> GGSKMEYEWKPDEQGLQQILQLLKESQSPDTTIQRTVQQKLEQLNQYPDFNNYLIFVLTKLKSEDEPTRSLSGLILKNNVKAHFQNFPNGVTDFIKSECLNNIGDSSPLIRATVGILITTIASKGELQNWPDLLPKLCSLLDSEDYNTCEGAFGALQKICEDSAEILDSDVLDRPLNIMIPKFLQFFKHSSPKIRSHAVACVNQFIISRTQALMLHIDSFIENLFALAGDEEPEVRKNVCRALVMLLEVRMDRLLPHMHNIVEYMLQRTQDQDENVALEACEFWLTLAEQPICKDVLVRHLPKLIPVLVNGMKYSDIDIILLKGDVEEDETIPDSEQDIRPRFHRSRTVAQQHDEDGIEEEDDDDDEIDDDDTISDWNLRKCSAAALDVLANVYRDELLPHILPLLKELLFHHEWVVKESGILVLGAIAEGCMQGMIPYLPELIPHLIQCLSDKKALVRSITCWTLSRYAHWVVSQPPDTYLKPLMTELLKRILDSNKRVQEAACSAFATLEEEACTELVPYLAYILDTLVFAFSKYQHKNLLILYDAIGTLADSVGHHLNKPEYIQMLMPP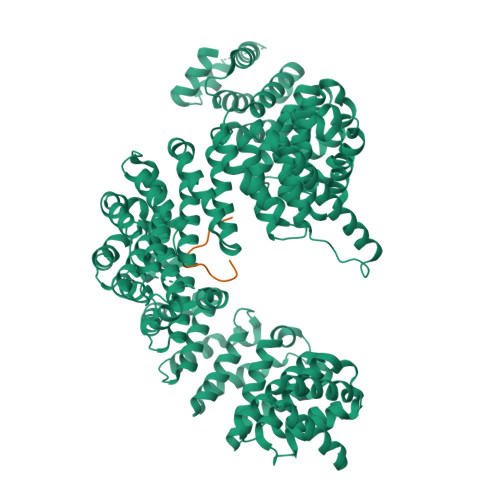LIQKWNMLKDEDKDLFPLLECLSSVATALQSGFLPYCEPVYQRCVNLVQKTLAQAMLNNAQPDQYEAPDKDFMIVALDLLSGLAEGLGGNIEQLVARSNILTLMYQCMQDKMPEVRQSSFALLGDLTKACFQHVKPCIADFMPILGTNLNPEFISVCNNATWAIGEISIQMGIEMQPYIPMVLHQLVEIINRPNTPKTLLENTAITIGRLGYVCPQEVAPMLQQFIRPWCTSLRNIRDNEEKDSAFRGICTMISVNPSGVIQDFIFFCDAVASWINPKDDLRDMFCKILHGFKNQVGDENWRRFSDQFPLPLKERLAAFYGV;> GGSNSPDTANDGFVRLRGLPFGCSKEEIVQFFSGLEIVPNGMTLPVDFQGRSTGEAFVQFASQEIAEKALKKHKERIGHRYIEIFKSSRAEVRTHYDPPRKLMAMQRPGPYDRPGAGRGYNSIGRG> RDQEQYIHRKCYQEFAHCYLVKYKTPQPWPNEGLIADQCPLPGLADVSFYPYQAIWDYYAKIENIRPANWTSSKLYGKARMGSYYIPKRLRNINNTHILFCSDVLYSKWYNLQNSILQNENELTKRLSNLTIGNKLKNRALPYEWAKGGLNRLFRNISVLDVCSRPEMVLLLNKTYYTFSLWEGDCNITRYNVNETVPECKDFPHRRFNDHPYSCRLWRYREGKEEVKCLTSDHTRCLYYPEYSNPEALFDFGFLSYMRNFPGPQCIESTSIRQQDYEVYSIYQECKLASKTYGIDSVLFSLKNFLNYTGKPVNEMPNARAFVGLIDPKFPPTYPDDDDK

The FV envelope (Env) glycoprotein belongs to a class I fusogens, which are synthesized as single-chain precursors that fold into trimers, and whose protomers are subsequently cleaved in the Golgi compartment during transport to the cell surface. FV Env is cleaved at two sites by cellular furin during maturation, giving rise to 3 fragments: the leader peptide (LP), the surface (SU) subunit, which includes the receptor-binding domain (RBD), and the transmembrane subunit (TM), which harbors the fusion machinery. In this manuscript we present the X-ray structure of the RBD from a zoonotic gorilla FV at 2.57 Å resolution, which reveals a novel fold. We identified, within the RBD, two subdomains in terms of their structure, conservation, and function: the upper subdomain, which encompasses most of the genotype-specific region, and a more conserved, lower subdomain, important for binding to the attachment factor HS.

Recombinant RBDs from several simian FV (SFV) strains were tested for production in Drosophila S2 insect cells, and only the RBD from gorilla SFV (strain SFVggo_huBAK7422, genotype II; abbreviated as ‘GII’ herein) was expressed in high enough yields and formed crystals. To increase the chances of generating well-diffracting crystals, a fraction of the purified protein was enzymatically deglycosylated (RBDD) with endoglycosidases H and D, as described in the Methods section. Crystals were obtained for the RBDD, as well as for the untreated protein (RBDG). The RBDD diffracted better (2.57 Å) than RBDG (2.80 Å) and the structural analyses presented below were carried out using the RBDD structure, unless otherwise noted. The upper subdomain forms a wider (~45 Å diameter) and the N- and C-termini a narrow lobe (~20 Å diameter), which is also termed lower subdomain. The lower subdomain is comprised of a three-helix bundle (α1, α7, α8) that packs against an antiparallel, twisted four-stranded β-sheet (β14-β1-β5-β15) and against helix α2 (residues 333-346) that lays perpendicularly on the side of the bundle. The upper subdomain is formed by two long excursions out of the lower subdomain: ~70 residues connecting strands β1 and β5, and ~130 residues connecting η4 and β14. The N390 side chain and the first two attached NAG residues are buried in the RBD, rendering the EndoH/D cleavage site inaccessible, which allowed building 10 sugar residues in RBDG and 8 in the deglycosylated protein crystals. The N8 glycan emerges from a cavity that has N390 at its base and extends upwards, remaining in contact with the protein and preserving the same conformation in both crystal forms. The 7 N-linked glycans that we could resolve in the RBDD structure are all fully solvent-exposed, and additional density was observed in the PFV EM map for the sugars attached to N5, N6, N7, N8, N9 and N11, validating the RBD placements (the N7’ site is absent from PFV Env, and no extra density was observed at this site).> GPHMTSDPVRQYLHEIGQVPLLTLEEEIDLARKVEEGMEAIKKLSEATGLDQELIREVVRAKILGTARIQKIPGLKEKPDPKTVEEVDGKLKSLPKELKRYLHIAREGEAARQHLIEANLRLVVSIAKKYTGRGLSFLDLIQEG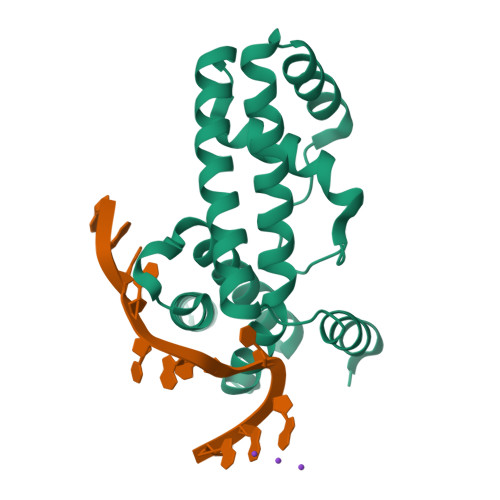NQGLIRAVEKFEYKRRFKFSTYATWWIRQAINRAIADQARTIRIPVHMVETINKLSRTARQLQQELGREPSYEEIAEAMGPGWDAKRVEETLKIAQEPVSL> GGCUUAUCAAGAGAGGUGAAGGGACUGGCCCGACGAAACCCGGCAACCAGAAAUGGUGCCAAUUCCUGCAGCGGAAACGUUGAAAGAUGAGCCGA

The SAM-I riboswitch contains an essential standard k-turn sequence that kinks a helix so that its terminal loop can make a long-range interaction. The SAM-I riboswitch is based around an elaborated four way helical junction; the crystal structure of the SAM-I riboswitch of Thermoanaerobacter tengcongensis was solved by Batey and colleagues, showing that the junction creates a pocket for the binding of SAM. Two adjacent helical arms of the junction make a tertiary contact in which the terminal loop of one helix (P2) base pairs with an internal loop within the other (P4). In order to do this, helix P2 must be severely kinked, and this is facilitated by a k-turn.

To address these questions, we have determined the crystal structure of the G2nA SAM-I riboswitch in complex with SAM. However, single-nucleotide substitutions at the second and third positions were less detrimental to ligand binding. The substitution G2nA prevented the folding of the isolated k-turn (see above). The same modification was introduced into the complete riboswitch, which was titrated with SAM. In contrast to the riboswitch modified at the 1b⋅1n position, the G2nA variant clearly bound SAM in an exothermic process, with thermodynamic parameters presented in Table 1. The corresponding binding affinity Kd = 0.31 ± 0.06 μM is similar to that of the natural riboswitch. The crystal was mounted on a cryoloop and diffracted to 2.6 Å. Turning to the k-turn region of the structure specifically, the natural and variant structures could be superimposed well (using the phosphorus atoms of residues 17–22 and 30–38), with an rmsd of 0.53 Å. Thus, the global fold of the variant k-turn is close to that of a standard k-turn structure, despite the presence of sequence changes that prevent folding of the same k-turn as an isolated duplex. The G2nA substitution creates a potential A⋅A base pair at the 2b⋅2n position, and we see that this pairing is stabilized by a single hydrogen bond from A2bN6 to A2nN3. The A⋅A pair is stacked between the G⋅A pairs at the 1b⋅1n and 3n⋅3b positions, both of which are standard trans sugar-Hoogsteen G⋅A pairs stabilized by hydrogen bonding between GN2 to AN7 and AN6 to GN3. The variant sequence forms an A⋅A pair at the 2b⋅2n position, held in place by a number of hydrogen bonds, and this study provides the first crystallographic structure of a standard k-turn with an A⋅A base pair at this position.>[6x]MKKIEAIIRPFKLDEVKIALVNAGIVGMTVSEVRGFGRQKGQTERYRGSEYTVEFL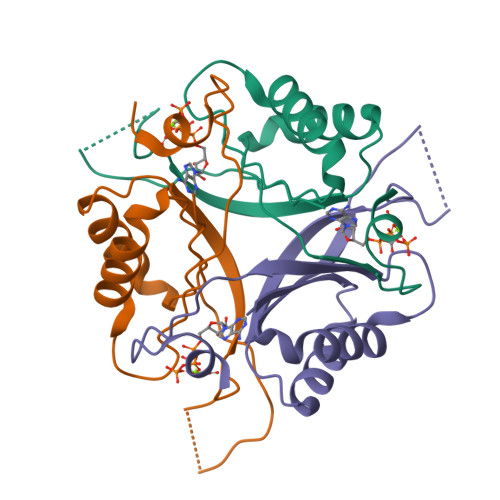QKLKLEIVVEDAQVDTVIDKIVAAARTGEIGDGKIFVSPVDQTIRIRTGEKNADAISAW> SMRKSREYEHVRRDLDPNEVWEIVGELGDGAFGKVYKAKNKETGALAAAKVIETKSEEELEDYIVEIEILATCDHPYIVKLLGAYYHDGKLWIMIEFCPGGAVDAIMLELDRGLTEPQIQVVCRQMLEALNFLHSKRIIHRDLKAGNVLMTLEGDIRLADFGVSAKNLKTLQKRDSFIGTPY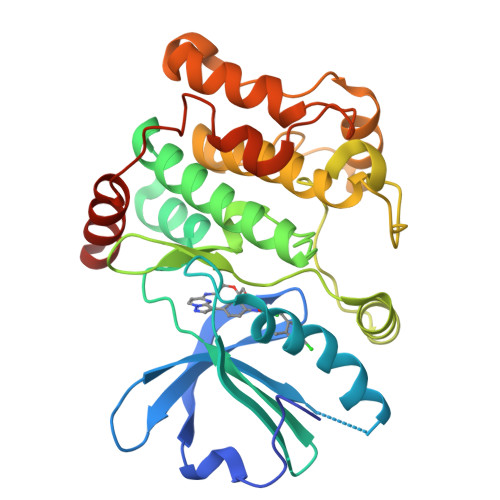WMAPEVVMCETMKDTPYDYKADIWSLGITLIEMAQIEPPHHELNPMRVLLKIAKSDPPTLLTPSKWSVEFRDFLAIALDKNPETRPSAAQLLEHPFVSSITSNKALRELVAEAKAEVMEE2'-DEOXY-5-NITROURIDINE 5'-(DIHYDROGEN PHOSPHATE) | C9 H12 N3 O10 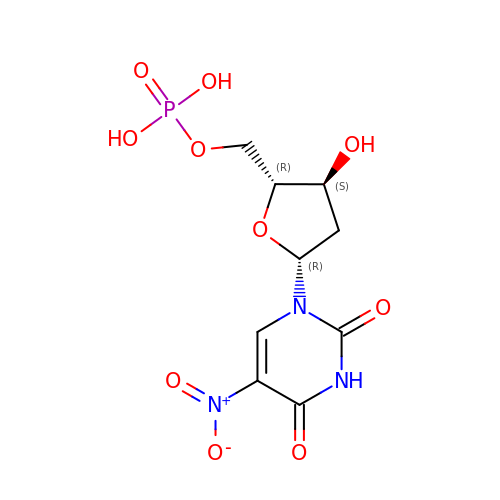P | LVLPVLNNXRTCHP-RRKCRQDMSA-N> GMVEVSQFKDAMAQLASAVHIVTTSGETGQHGFTASAVCSVTDSPPTLLVC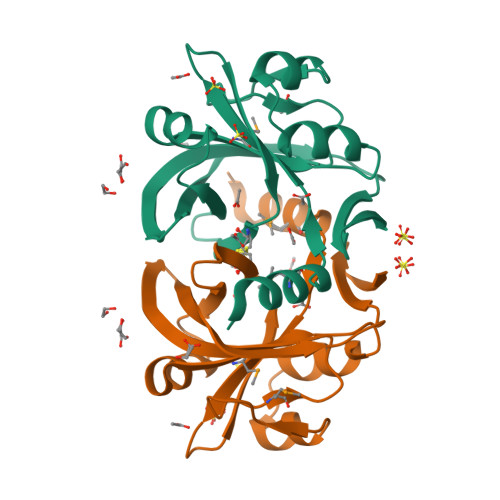INSNARAYEHFVKNRVLMVNTLTAEQSSLSNIFASPLSQEERFSNASWTTLTTGSPMLQDALINFDCEITEIKHVGTHDILICKIVDIHQSNAKNALVYRNRVYHSV Fatty acid-binding proteins (FABPs) are involved in the uptake, metabolism and intracellular trafficking of fatty acids. Based on epidemiological studies and animal knockout models, the isoforms FABP4 and FABP5 were identified as potential diabetes and atherosclerosis targets. The aim of this study was to develop a dual FABP4/5 inhibitor and, to this end, high-throughput and fragment screens were conducted with X-ray crystallography as a follow-up method on those ligands that showed appreciable affinity and favorable physicochemical properties. Structure-based drug design (SBDD) based on initial hits from high-throughput and fragment screens yielded 216 ligand-bound structures of human FABP3, FABP4 and FABP5 isoforms, many of which were at resolutions of better than 1.2 Å.

During this exercise, 229 FABP crystal structures from various human and mouse isoforms were determined, many at better than 1.2 Å resolution.

>[4x]GSHMASLKDLEGKWRLMESHGFEEYMKELGVGLALRKMAAMAKPDCIITCDGNNITVKTESTVKTTVFSCNLGEKFDETTADGRKTETVCTFQDGALVQHQQWDGKESTITRKLKDGKMIVECVMNNATCTRVYEKVQ> SNAMADKKATLHVEGKAPIELPIMEGSLGTPVIDVRKLGANGYFTFDPGFLATASCESQITYIDGGKGILLHRGYPIDQLANNADYLEVCYILLYGEAPTREQYEKFKTTVTRHTMVHEQIASFFHGFRRDAHPMAVMCGVVGALAAFYHDSLDINNDLHREITAYRLLSKMPTLAAMCYKYSTGQPFIYPRNDLSYAENFLHMMFATPCEEYEVNPVVARAMDKIFTLH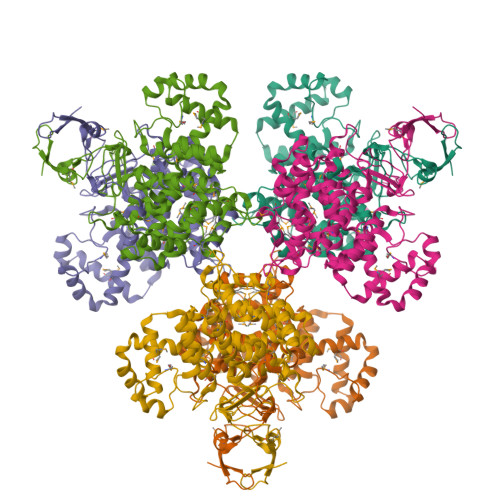ADHEQNASTSTVRLAGSSGANPFACIAAGIASLWGPAHGGANEACLKMLEEIGSVDNIPEYVDRAKDKDDPFRLMGFGHRVYKNYDPRATVMRETCHEVLKELNIQDPLLDVAMELERIALSDEYFVSKKLYPNVDFYSGIILKAIGIPVSMFTVIFAISRTIGWIAHWNEMHSDPLNRIGRPRQLYTGEVQRDFQPMHERE>[2x]MGHHHHHHENLYFQGHMTPELRAKLESLGRDLTPEMLGGTTQIFAAMATGSDPEVEVTRDLEYGEDPRHRL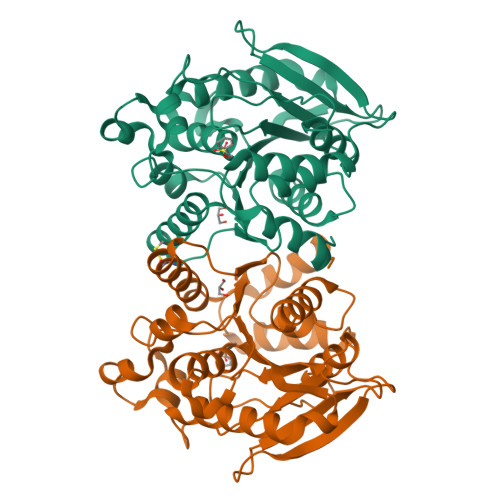DLFRKADTRDAPVLVFVHGGGFVMGDKRLAETPFYDNIGVFAAQQGFVGVTITYRLAPAHQFPSGPEDLAAVVRWLKANVAQYGGDPDKIVLSGQSAGAAHVASYIAHKAHHATEGGGIAGAILMSGIYDTLTATPNEFLIAYYGDDPKGWGPASSMAGLINTEIPLMLTVSEFDPEDFQRQAAQFVCAWGMAHAAYPEMHYLVGHNHLSPAQSIGTEIKAIGRMVAGFVRRVTR> YYKE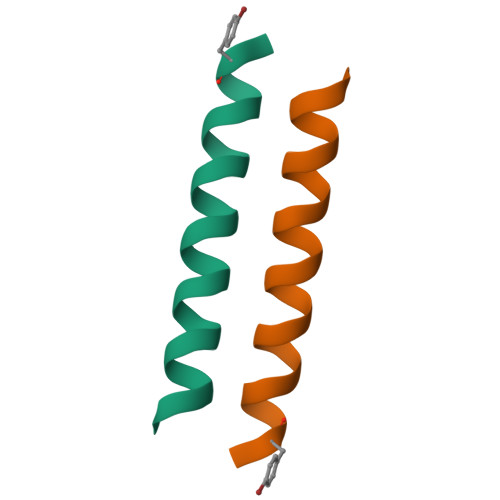IAHALFSALFALSELYIAVRYX> QLIFDDCVFA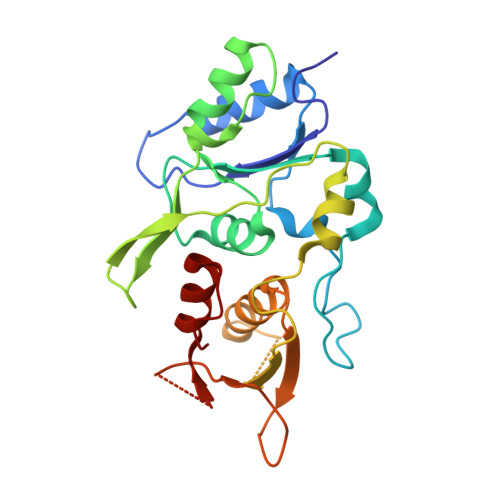FSGPVHEDAYDRSALETVVQDHGGLVLDTGLRPLFNDPFKSKQKKLRHLKPQKRSKSWNQAFVVSDTFSRKVKYLEALAFNIPCVHPQFIKQCLKMNRVVDFSPYLLASGYSHRLDCTLSQRIEPFDTTDSLYDRLLARKGPLFGKKILFIIPEAKSWQKKIENTEQGQKALAHVYHALALGADVEIRPNVAHLECDLILTMDGNIVDETNCPVVDPEWIVECLISQSDIST> TARIALASLFVVAAVLAQPWQTTTQRWVLGVSIAAVIVLLAWWKGMFLTTRIGRALAMVRRNRAEDTVETDAHRATVVLRVDPAAPAQLPVVVGYLDRYGITCDKVRITHRDAGGTRRSWISLTVDAVDNLAALQARSARIPLQDTTEVVGRRLADHLREQGWTVTVVEGVDTPLPVSGKETWRGVADDAGVVAAYRVKVDDRLDEVLAEIGHLPAEETWTALEFTGSPAEPLLTVCAAVRTSDRPAAKAPLAGLTPARGRHRPAL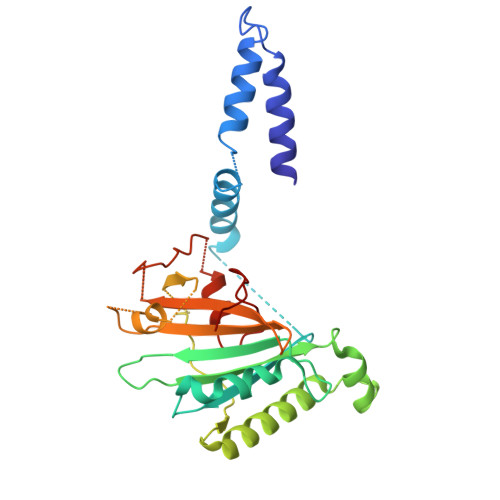AALNPLSTERLDGTAVPLPA> MSDLIEYSFYLTYAFLMTTGTITFIEALRTKNESVRHILNLETCISVVAAFFYSNFIGKLEHINYEEINLNRYVDWAITTPIMLLVLVLAFRVNQTNKAMVKFSDFMIIL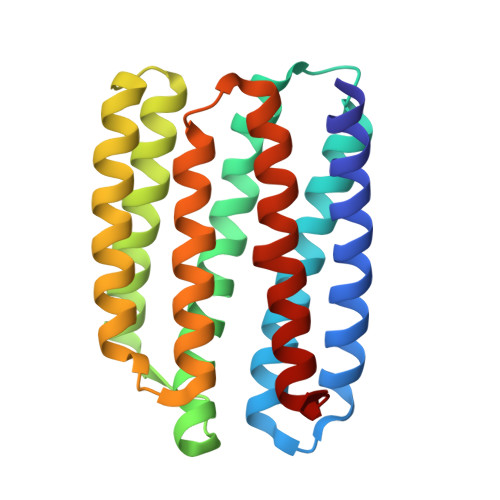GMNYGMLGTGYLGDIGVIHKTMGTVLGFLFFGGLFYKLNTLRTSNASNDLLYGAFFVLWALYGVFYQMEQLPRNVGYNVLDLFSKCFVGIYFWAFYAKIFT>SAHPYLIQRLGIEQGLSNNYVLSITQDKQGFLWFATEEGLNKFDGTRFITYYKEEQSSSVQSITGNELNEVYTDPVQPVIWIATQRAGLNAYNYETQSFSVYQYNPEDPQSLITNDVTHITSSVQAGKGLWVCTYYRGIEYLDIATGKFTHYNKSTVPALPSEQTWTATEAEDGKLYIGHVEGGLSILSLNDKSVKHFVHDPQNPNSLPGNDVRCIYKDTNGNIWIGTSKGLALFNANTETFTNFHNNPGNIHGALSSYIFSIKQLKDNKLWIATELNGIMILDLQQNQFLLPEQIRFEFIREGDNNYSLSNASARYIFQDSFNNIWIGTWGGGINFISNAPPTFHTWSYSPTQMNESSLSNKVVSSVCDDGQGKLWIGTDGGGINVFENGKRVAIYNKENRELLSNSVLCSLKDSEGNLWFGTYLGNISYYNTRLKKFQIIELEKNELLDVRVFYEDKNKKIWIGTHAGVFVIDLASKKVIHHYDTSNSQLLENFVRSIAQDSEGRFWIGTFGGGVGIYTPDMQLVRKFNQYEGFCSNTINQIYRSSKGQMWLATGEGLVCFPSARNFDYQVFQRKEGLPNTHIRAISEDKNGNIWASTNTGISCYITSKKCFYTYDHSNNIPQGSFISGCV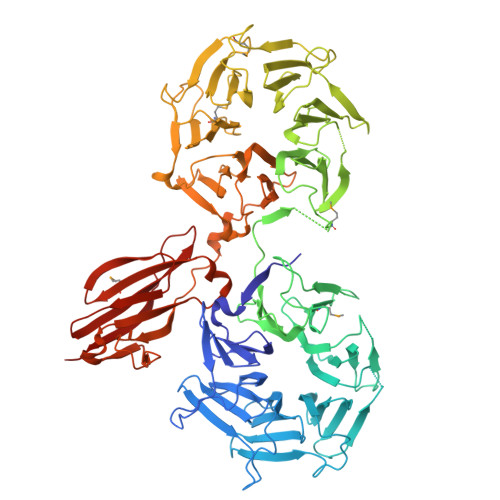TKDHNGLIYFGSINGLCFFNPDIAINSPQIPPVVITKVRIPGRLTSREKNETAIPISEGEIELTHEQNSFNLTFNVQDYSLANQVEYAYMLKGLENSWYTINEQNSVTFRNIPPGKYEFLVKARLHNQDWSEDTTSLRIHINPPLWLT[4x]(1R,3S,4S,5R,6S)-2,4,5,6-tetrakis(phosphonooxy)cyclohexane-1,3-diyl bis[trihydrogen (diphosphate)] | C6 H20 O30 P8 | 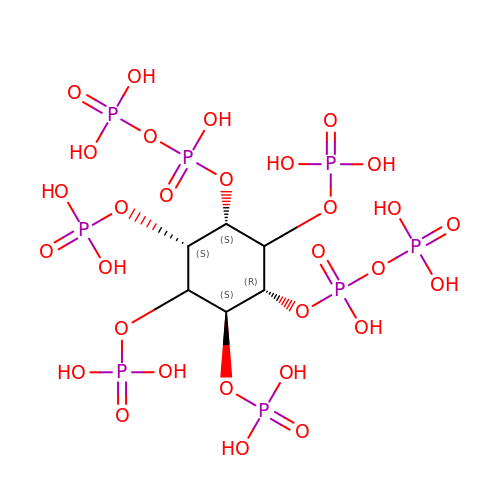HHQOOERQSFJGEP-ZSIQDKGESA-N>AMDPEFETGEVVDCHLSDMLQQLHSVNASKPSERGLVRQEEAEDPACIPIFWVSKWVDYSDKYGLGYQLCDNSVGVLFNDSTRLILYNDGDSLQYIERDGTESYLTVSSHPNSLMKKITLLKYFRNYMSEHLLKAGANITPREGDELARLPYLRTWFRTRSAIILHLSNGSVQINFFQDHTKLILCPLMAAVTYIDEKRDFRTYRLSLLEEYGCCKELASRLRYARTMVDKLLSSRSASNRLKAS[2x];>WSSSLATPPTLSSTVLI[2x]

The BRCA2 tumor suppressor protein plays an important role in DNA repair by homologous recombination (HR)1,2 that takes place preferentially during S/G2 phases of the cell cycle. PLK1 is a master regulator of the cell cycle that is upregulated in mitosis. PLK1 is recruited to specific targets via its Polo-box domain (PBD). PBD interacts with phosphosites characterized by the consensus motif S-[pS/pT]-P/X23.

Here, we demonstrate that the two conserved residues S193 and T207 are phosphorylated by PLK1, and that phosphorylated BRCA2-T207 is a bona fide docking site for PLK1. To demonstrate the recognition of pT207 by PLK1, we measured the affinity of recombinant PLK1PBD (the target recognition domain of PLK1) for a synthetic 17 aa peptide comprising phosphorylated T207. Using isothermal titration calorimetry (ITC), we found that recombinant PLK1PBD bound to the pT207 peptide with an affinity of Kd = 0.09 ± 0.01 µM, similar to the optimal affinity reported for an interaction between PLK1PBD and its phosphorylated target. A peptide comprising pT207 and the mutation S206C could not bind to PLK1PBD, as predicted from the consensus sequence requirement for PLK1PBD interaction. Finally, we determined the crystal structure of PLK1PBD bound to the T207 phosphorylated peptide at 3.1 Å resolution. Analysis of this 3D structure showed that, as expected, the 17 aa BRCA2 phosphopeptide binds in the cleft formed between the two Polo boxes. Twelve residues of the peptide (from A199 to I210) are well structured upon binding, burying about 694 Å2 in the interface with PLK1PBD. The interface between BRCA2 and PLK1PBD is stabilized by 12 hydrogen bonds: the backbone of residues T200 to L209 as well as the side chain of S206 are bonded to residues from Polo Box 1, whereas the side chain of phosphorylated T207 is bonded to residues from Polo Box 2 (see the zoom view in Fig. 3l). The side chain of S206 participates in two hydrogen-bonding interactions with the backbone of W414, which explains the strict requirement for this amino acid at this position. Moreover, the phosphate group of pT207 participates in three hydrogen-bonding interactions with the side chains of residues H538, K540, and R557 in Polo Box 2 (see the zoom view in Fig. 3l).2-PROPYLPENTANAMIDE | C8 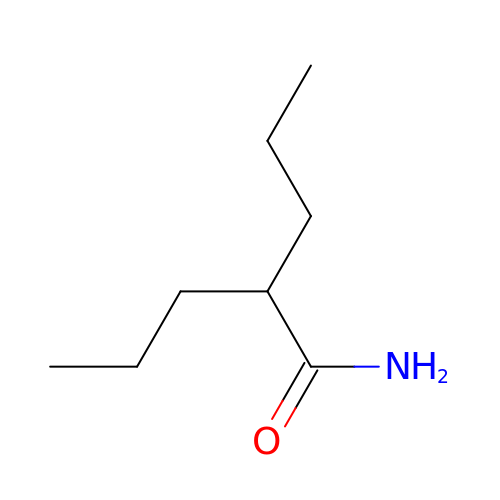H17 N O | OMOMUFTZPTXCHP-UHFFFAOYSA-N>[2x]MGSSHHHHHHSSGRENLYFQGMPKLILASTSPWRRALLEKLQISFECAAPEVDETPRSDESPRQLVLRLAQEKAQSLASRYPDHLIIGSAQVCVLDGEITGKPLTEENARLQLRKASGNIVTFYTGLALFNSANGHLQTEVEPFDVHFRHLSEAEIDNYVRKEHPLHCAGSFKSEGFGITLFERLEGRDPNTLVGLPLIALCQMLRREGKNPLMG

Maf (for multicopy associated filamentation) proteins represent a large family of conserved proteins implicated in cell division arrest but whose biochemical activity remains unknown. Here, we show that the prokaryotic and eukaryotic Maf proteins exhibit nucleotide pyrophosphatase activity against 5-methyl-UTP, pseudo-UTP, 5-methyl-CTP, and 7-methyl-GTP, which represent the most abundant modified bases in all organisms, as well as against canonical nucleotides dTTP, UTP, and CTP. The protomer structures of the four Maf proteins revealed a large β sheet containing seven β strands (β1 to β7) with two α-helical subdomains on one side and one long α helix on another side. Thus, pyrophosphatase activity of Maf proteins toward canonical and modified nucleotides might provide the molecular mechanism for a dual role of these proteins in cell division arrest and house cleaning.

Screening of Maf proteins for pyrophosphatase activity against a set of 57 noncanonical or modified nucleoside triphosphates revealed that the YhdE-like Maf proteins (E. coli YhdE, BSU28050, YOR111W, and ASMTL-Maf) also exhibited high pyrophosphatase activity against 5-methyl-UTP (m5UTP or riboTTP), pseudouridine triphosphate (pseudo-UTP or Ψ), and 5-methyl-CTP (m5CTP), whereas the two YceF proteins (from E. coli and S. typhimurium) were active toward 7-methyl-GTP (m7GTP). The Michaelis-Menten constant, KM, of the YhdE-like proteins toward canonical pyrimidine nucleotides varied in a micromolar range: 32.7–53.0 μM for dTTP; 29.7–72.4 μM for UTP; and it was lower (to a lesser extent for ASMTL-Maf) with modified nucleotides (4.7–47.2 μM). Both YceF proteins also showed high affinity to m7GTP (32.8 μM for YceF and 30.9 μM for STM1189). Therefore, we propose that the unprotonated Asp88 of ASMTL-Maf (Asp70 in YhdE, Asp103 in YOR111W, Asp70 in BSU28050, and Asp69 in YceF) functions as a general base coordinating a water molecule to produce a nucleophilic hydroxide ion, which attacks the alpha-phosphate of the substrate. This is supported by the complete loss of activity in the ASMTL-Maf D88A (and D88N), YhdE D70A, YOR111W D103A, BSU28050 D70A, and YceF D69A mutant proteins. The structure of the inactive YceF D69A protein showed no changes in the position of the side chains of other residues in the active sites, suggesting that the loss of activity in this protein is caused by the replacement of the catalytic Asp69 by Ala. Alanine replacement mutagenesis of the predicted triphosphate binding residues in ASMTL-Maf (Arg24, Lys65, Lys100), YOR111W (Arg30, Lys74, Lys116), YhdE (Arg13, Lys52, Lys82), BSU28050 (Arg14, Lys53, Lys82), and YceF (Arg13, Lys52, Lys81) produced inactive proteins, confirming that these residues play an important role in activity of Maf proteins and suggesting that they are likely to be involved in the coordination of the triphosphate part of the substrate.>[4x]T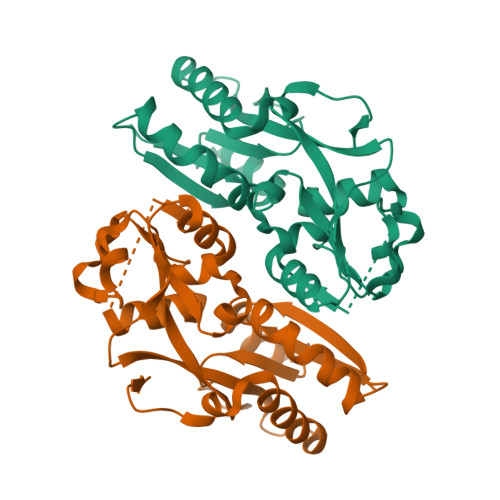GRLNIAVLPTIAPYLLPRVFPIWKKELAGLEIHVSEMQTSRCLASLLSGEIDMAIIASKAETEGLEDDLLYYEEFLGYVSRCEPLFEQDVIRTTEVNPHRLWLLDEGHSFRDQLVRFCQMKGLHERQTAYSGGSMEAFMRLVESGQGITFIPQLTVEQLSPSQKELVRPFGMPRPVREVRLAVRQDYSRRKLREQLIGLLRSAVPSDMHKLQTGQHLAHHHH>[4x]MGFLVMIREVSMAKAIRVVLLCVSVLWVVPKECACRSNFSRNSSSSSSSSLRPLRQRPSSVNVGALFTYDSFIGRAAKPAVKAAMDDVNADQSVLKGIKLNIIFQDSNCSGFIGTMGALQLMENKVVAAIGPQSSGIAHMISYVANELHVPLLSFGATDPTLSSLQFPYFLRTTQNDYFQMHAIADFLSYSGWRQVIAIFVDDECGRNGISVLGDVLAKKRSRISYKAAITPGADSSSIRDLLVSVNLMESRVFVVHVNPDSGLNVFSVAKSLGMMASGYVWIATDWLPTAMDSMEHVDSDTMDLLQGVVAFRHYTIESSVKRQFMARWKNLRPNDGFNSYAMYAYDSVWLVARALDVFFRENNNITFSNDPNLHKTNGSTIQLSALSVFNEGEKFMKIILGMNHTGVTGPIQFDSDRNRVNPAYEVLNLEGTAPRTVGYW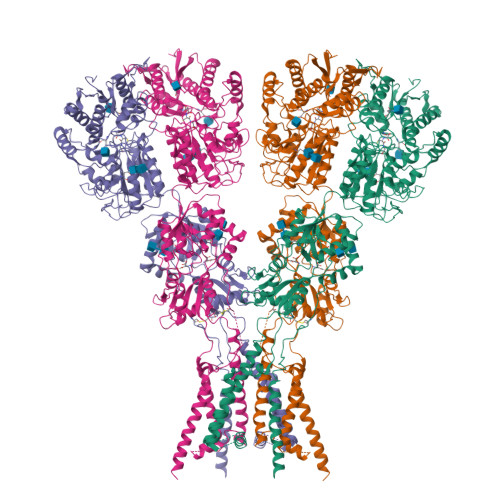SNHSGLSVVHPETLYSRPPNTSTANQRLKGIIYPGEVTKPPRGWVFPNNGKPLRIGVPNRVSYTDYVSKDKNPPGVRGYCIDVFEAAIELLPYPVPRTYILYGDGKRNPSYDNLVNEVVADNFDVAVGDITIVTNRTRYVDFTQPFIESGLVVVAPVKEAKSSPWSFLKPFTIEMWAVTGGFFLFVGAMVWILEHRFNQEFRGPPRRQLITIFWFSFSTMFFSHRENTVSSLGRFVLIIWLFVVLIINSSYTASLTSILTIRQLTSRIEGIDSLVTSNEPIGVQDGTFARNYLINELNILPSRIVPLKDEEQYLSALQRGPNAGGVAAIVDELPYIEVLLTNSNCKFRTVGQEFTRTGWGFAFQRDSPLAVDMSTAILQLSEEGELEKIHRKWLNYKHECSMQISNSEDSQLSLKSFWGLFLICGITCFMALTVFFWRVFWQYQRLLPESADEERAGEVSEPSRSGRGSRAPSFKELIKVVDKREAEIKEILKQKSSKKLKSTQSAAGTSQSQHGEIT>[2x]MEQRRGDSMAGGAPAEDGYNWRKYGQKLVK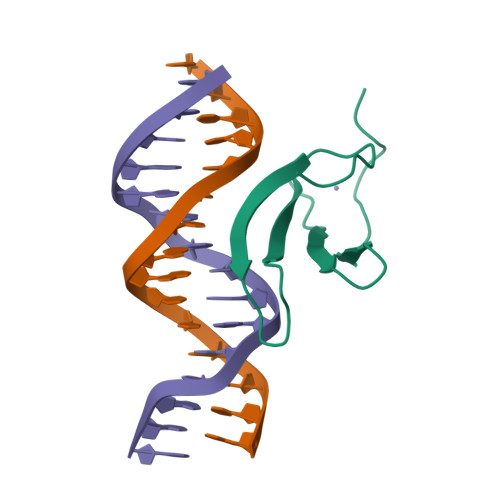GSEYPRSYYKCTNPNCQVKKKVERSREGHITEIIYKGAHNHLKPLEHHHHHH> MSHHKKRVYPQAQLQYGQNATPLQQPAQFMPPQDPAAAGMSYGQMGMPPQGAVPSMGQQQFLTPAQEQLHQQIDQATTSMNDMHLHNVPLVDPNAYMQPQVPVQMGTPLQQQQQPMAAPAYGQPSAAMGQNMRPMNQLYPIDLLTELPPPITDLTLPPPPLVIPPERMLVPSELSNASPDYIRSTLNAVPKNSSLLKKSKLPFGLVIRPYQHLYDDIDPPPLNEDGLIVRCRRCRSYMNPFVTFIEQGRRWRCNFCRLANDVPMQMDQSDPNDPKSRYDRNEIKCAVMEYMAPKEYTLRQPPPATYCFLIDVSQS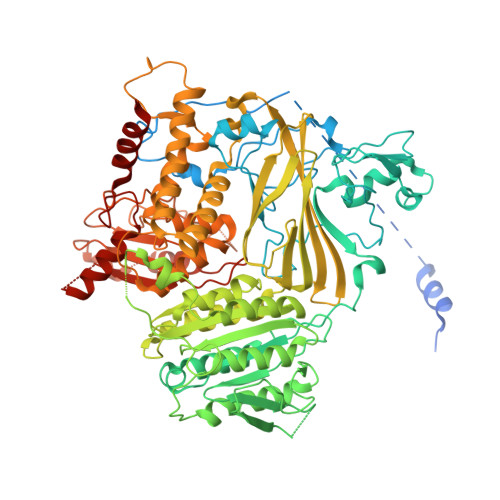SIKSGLLATTINTLLQNLDSIPNHDERTRISILCVDNAIHYFKIPLDSENNEESADQINMMDIADLEEPFLPRPNSMVVSLKACRQNIETLLTKIPQIFQSNLITNFALGPALKSAYHLIGGVGGKIIVVSGTLPNLGIGKLQRRNESGVVNTSKETAQLLSCQDSFYKNFTIDCSKVQITVDLFLASEDYMDVASLSNLSRFTAGQTHFYPGFSGKNPNDIVKFSTEFAKHISMDFCMETVMRARGSTGLRMSRFYGHFFNRSSDLCAFSTMPRDQSYLFEVNVDESIMADYCYVQVAVLLSLNNSQRRIRIITLAMPTTESLAEVYASADQLAIASFYNSKAVEKALNSSLDDARVLINKSVQDILATYKKEIVVSNTAGGAPLRLCANLRMFPLLMHSLTKHMAFRSGIVPSDHRASALNNLESLPLKYLIKNIYPDVYSLHDMADEAGLPVQTEDGEATGTIVLPQPINATSSLFERYGLYLIDNGNELFLWMGGDAVPALVFDVFGTQDIFDIPIGKQEIPVVENSEFNQRVRNIINQLRNHDDVITYQSLYIVRGASLSEPVNHASAREVATLRLWASSTLVEDKILNNESYREFLQIMKARISK>MGSSHHHHHHSSGLVPRGSTSEVIEDEKQFYSKAKTYWKQIPPTVDGMLGGYGHISSIDINSSRKFLQRFLREGPNKTGTSCALDCGAGIGRITKRLLLPLFREVDMVDITEDFLVQAKTYLGEEGKRVRNYFCCGLQDFTPEPDSYDVIWIQWVIGHLTDQHLAEFLRRCKGSLRPNGIIVIKDNMAQEGVILDDVD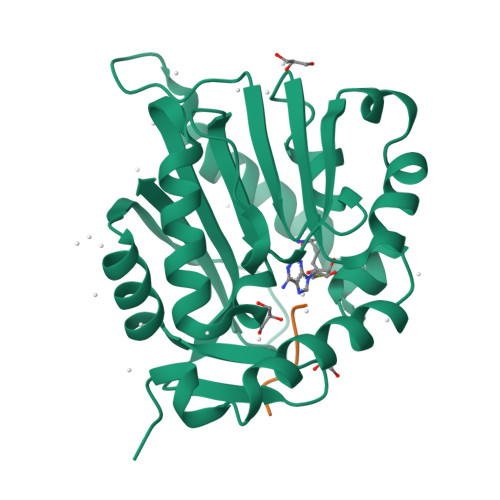SSVCRDLDVVRRIICSAGLSLLAEERQENLPDEIYHVYSFALR[2x];>[2x]SPKRIA>GSHMRIAQVAPLWERVPPPAYGGVELVVSLLTEELVKRGHEVTLFASGDSMTQAKLVSTYPHAIR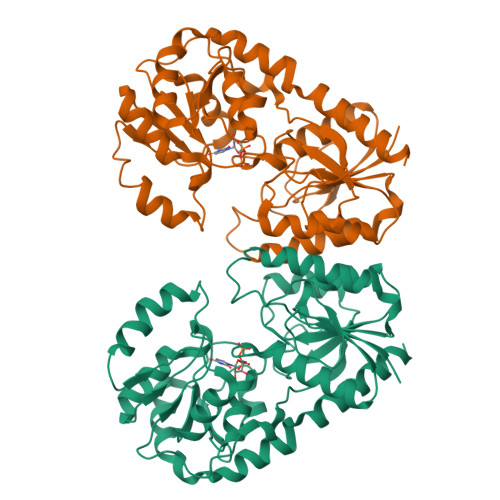LDPNVQEYAVYEALQLGEVFSRANEFDVIHSHVGYTALPYTSLVKTPVVHTLHGRFTADNERIFSQYRNQNYVSISHSQRQLRELNYIATVYNAIAVETHHFYPQPSDPPYLAFLGRLSPEKGPHHAIEIAKRVGIPLRMAGKVDRVDRDYFKELIEPHIDGEFIQFIGEADHPTKNALLGGAIAMLFPITWQEPFGLVMIESMAAGTPVVAIAKGAAPEVIEHGKTGFLCHSVEDCVAAVAQVPQLDRMACRDYVWQRFSVERMVSEYEAVYDTVLANTFVHNGHRRGTIELMAS[2x]> SVDHGFLVTRHSQTIDDPQCPSGTKILYHGYSLLYVQGNERAHGQDLGTAGSCLRKFSTMPFLFCNINNVCNFASRNDYSYWLSTPEPMPMSMAPITGENIRPFISRCAVCEAPAMVMAVHSQTIQIPPCPSGWSSLWIGY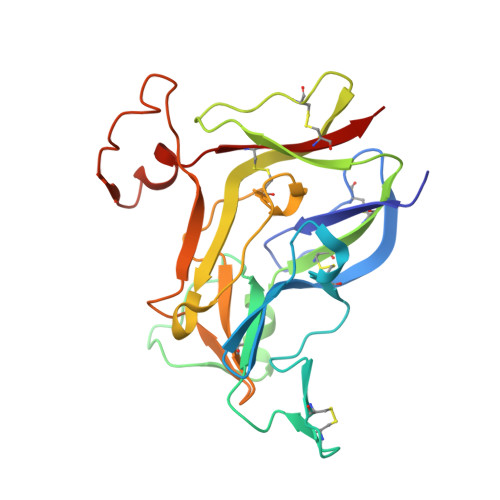SFVMHTSAGAEGSGQALASPGSCLEEFRSAPFIECHGRGTCNYYANAYSFWLATIERSEMFKKPTPSTLKAGELRTHVSRCQVCMRRT> MKSESKVSSKLELRELVLLAMVIAIKVILGQFKVGNATLQVGLGFIGSVMLGYLFGPWWGFAGGALSDLVSSVIFGNLGGFFIGFTLTAALGPMIYGFFLYKQPIQIWRVIASVICVTVICNIGLNTLWVSMMYGINFMVALSSRILKE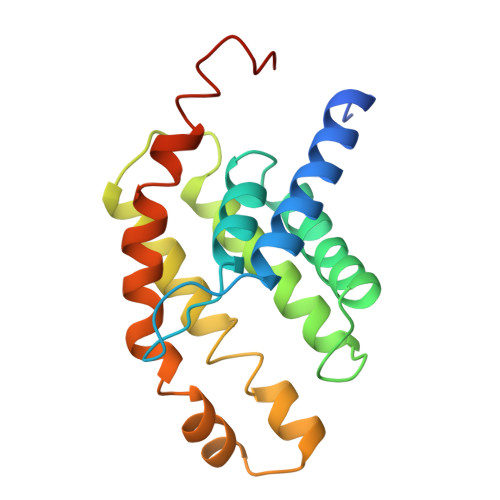MITPWIQMVAVWFILEGLSRVKLSRKFWSHPQFEK1-DECANE-SULFONIC-ACID | C10 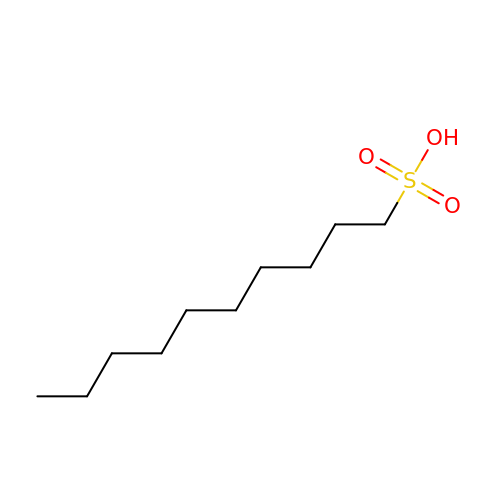H22 O3 S | KVGOXGQSTGQXDD-UHFFFAOYSA-N> GSSHHHHHHSSGLVPRGSHMGSIIDAAAAAGPVVLMETAFRKAVESRQIPGAVIMARDASGNLNYTRCFGARTVRRDENNQLPPLQVDTPCRLASATKLLTTIMVLQCMERGLVDLDETVDRLLPDLSAMPVLEGFDDAGNARLRERRGKITLRHLLTHTSGLSYVFLHPLLREYMAQGYLQSAEKFGIQSRLAPPAVNDPGAEWIYGTNLDWAGKLVERATGLDLEQYLQENICAPLGITDMTFKLQQRPDMLARRADQTHRNSADGRLRYDDSVYFRADGEECFGGQGVFSSPGSYMKVLHSLLKRDGLLLQPQTVDLMFQPALEPRLEEQMNQHMDASPHINYGGPMPMVLRRSFGLGGIIALED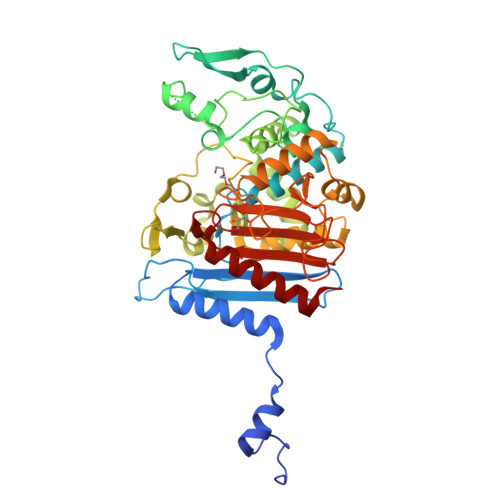LDGENWRRKGSLTFGGGPNIVWQIDPKAGLCTLAFFQLEPWNDPVCRDLTRTFEHAIYAQYQQG>MIITVTLNMEKYNFLGISIVGQSNERGDGGIYIGSIMKGGAV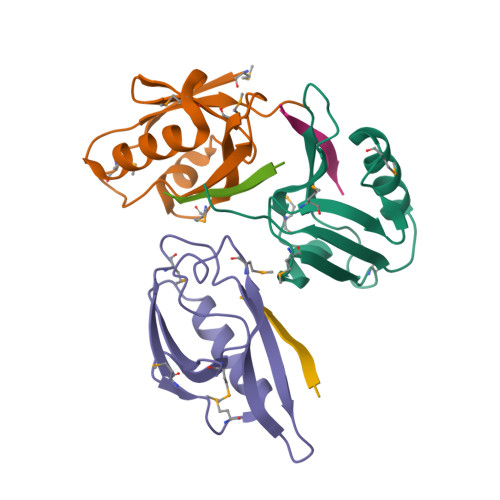AADGRIEPGDMLLQVNDINFENMSNDDAVRVLRDIVHKPGPIVLTVAKLEHHH[3x];>[3x]SLKLMTTV>CPGIVPRSVWGARETHCPRMTLPAKYGIIIHTAGRTCNISDECRLLVRDIQSFYIDRLKSCDIGYNFLVGQDGAIYEGVGWNVQGSSTPGYDDIALGITFMGTFTGIPPNAAALEAAQDLIQCAMVKGYLTPNYLLV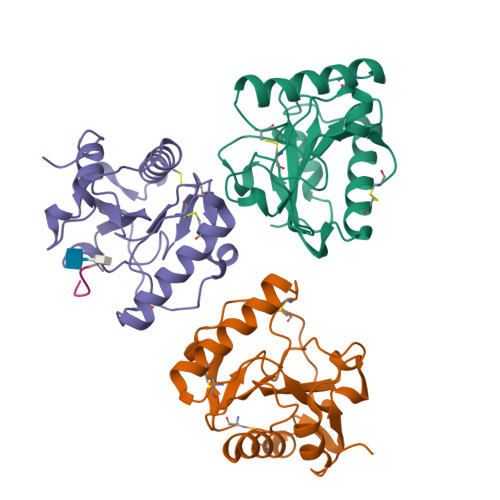GHSDVARTLSPGQALYNIISTWPHFKH[3x];> AEKAA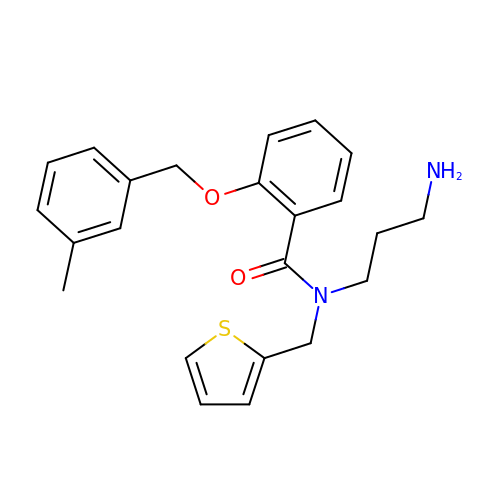N-(3-aminopropyl)-2-[(3-methylphenyl)methoxy]-N-[(thiophen-2-yl)methyl]benzamide | C23 H26 N2 O2 S | LCQJRANJHOEQFG-UHFFFAOYSA-N>[4x]HHSAGCPSQCSCDQTL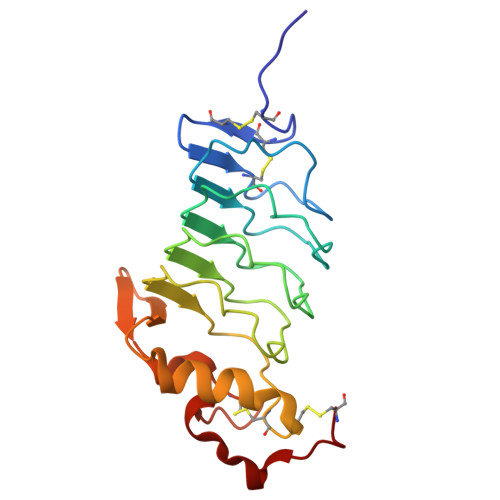VNCQNIRLASVPAGIPTDKQRLWLNNNQITKLEPGVFDHLVNLQQLYFNSNKLTAIPTGVFDKLTQLTQLDLNDNHLKSIPRGAFDNLKSLTHIYLYNNPWDCECRDIMYLRNWVADHTSIVMRWDGKAVNDPDSAKCAGTNTPVRAVTEASTSPSKC>MNIQAIDTRHGTANQHSFSNGNCLPYTGVPFGMNFYAPQTTDQKGSWWFHPEDRTFQGYRVTHQPSPWMGDFSHLLMTPVSGSLSELSLFHAQSSYRPEESLFSPVEINLTQLRYQITSQLIPSMYGGILTIDYQQKDNHLLLTLPGRYQVKQLDDHQVAVKVINYSGCEDPDFSFYFVLHFEQPLTKWFAPSSGEDGKILLSFGNIAQQVVHFSSSFISEKQAQLNLAREISLRSTEMLQQGIADWHNYFDRLKVTHENPEHTKTFYHTLYRTFLFPQTFYELDENQQPIHYDTFSQTVRPGVLYTNNGFWDTYKTVYPLFSLIAQEKYEEMLEGFLNSYNETGFLPKWLSPDERGLMPGTLIDAVIADAAVKKIRPDLMPQFLEAMKKGATQQSERENYGRQGTLDYLKYGYVPSTYHESVNHTLDYAYSDFCISQVAKTLNDSETATFYRQQALNYQQLFNPETGFMQAKDTEGNFRPDFLDIRWGKDYAQGSAWQSSFAVYQDFAGLIKLYGSELAFEKKLIQLCNQAPNFNVEGYGFEIHEMSEMAA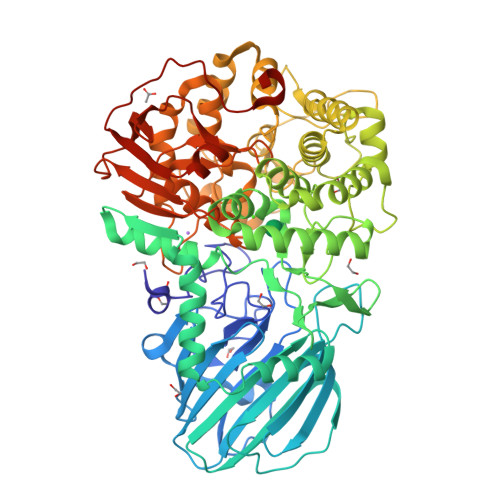IDFGQLAISNQPSFHYPFLFSYIGKPEMAQPLLKQLMQTFDASPTGYPGDEDNGSMSAWYIFNSLGFYPVTPGAGEYVIGMPLVQTAEVKLSNGKQLTIQTSPNKVQQQFIHEIQLNQEKHTAPYFTHQELLNGGTLDYQLGIVPNPQTTAERPFSLSTEKLEHHHHHH[4x]>[2x]GSHMDPGTVLEISRSLKKRMQDILKKDNANNLEGRPATGKIENVEEISDILMSKALQESLLDEGILDEIKGWLEPLPDKSMPNIKIRKRLLDVLKTMKIHKEHLVTSGVGKIVYFYSI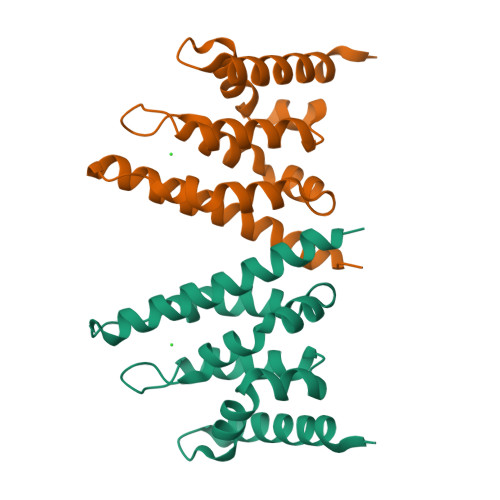NPKESKEVRASAKALVQKWTNEVFKPEGGD> MHHHHHHEENVKRRTHNVLERQRRNELKRSFFALRDQIPELENNEKAPKVVILKKATAYILSVQAEE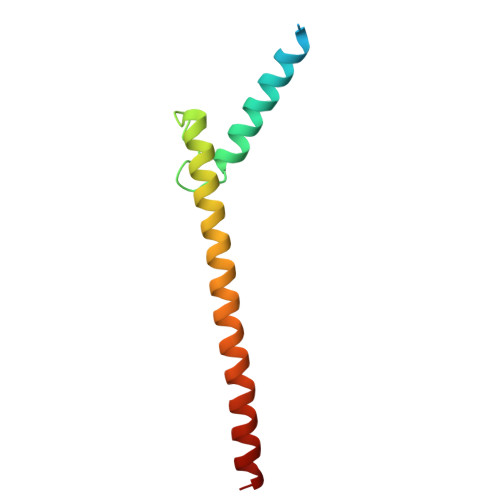QKLISEEDLLRKRREQLKHKLEQLRNS>[2x]MHHHHHHMLENKLGIINQLELNRVEERVSKENAKRLYD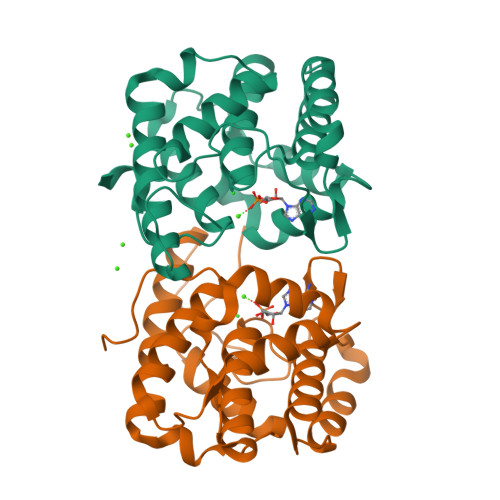SGDIDRIEVGTFKGLSYIHNYLFEDIYEFAGKVRSQNISKGNFRFAPVMYLEIALEHIDKMPQRNLDEIVAKYVEMNIAHPFREGNGRATRIWLDLILKKELKRVVDWNLINKEDYLSAMERSPVKDLEIKYLISNALTDKINDREIFMKGIDISYYYEGYTEYNVDEL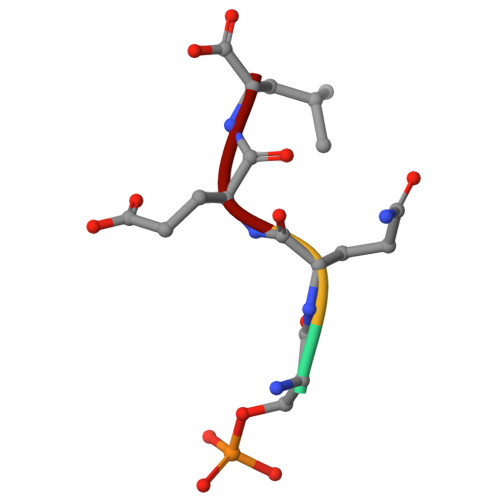> SQEL> MKNVYLPITVDHIARVE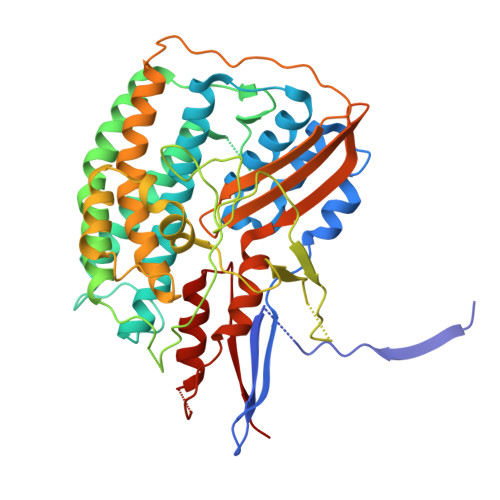GKGGVEIVVGDDGVKEVKLNIIEGPRFFEAITLGKKLDEALAIYPRICSFCSAAHKLTAVEAAEKAIGFTPREEIQALREVLYIGDMIESHALHLYLLVLPDYLGYSGPLHMIDEYKKEMSIALDLKNLGSWMMDELGSRAIHQENAVLGGFGKLPDKSVLENMKRRLKEALPKAEYTFELFTKLEQYEEVEGPITHIAVKPRNGVYGIYGDYLKASDGNEFPSEEYREHIKEFVVEHSFAKHSHYHGKPFMVGAISRLVNNADTLYGRAKELYESYKDLLRSTNPFANNLAQALELVYFTERAIDLIDEALAKWPIRPRDEVALKDGFGVSTTEAPRGVLVYALKVENGRVSYADIITPTAFNLAMMEQHVRMMAEKHYNDDPEKLKLLAEMVVRAYDPCISCSVHVARL> SPLQAKKVR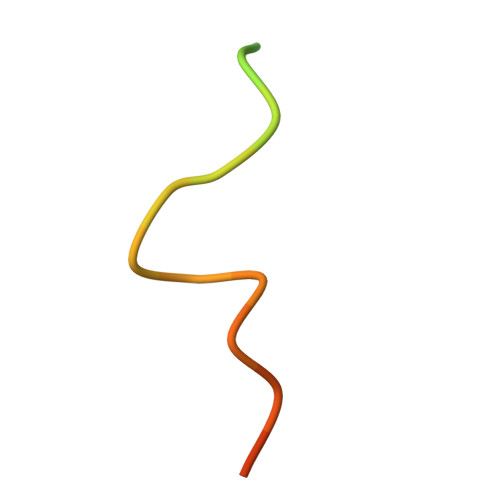KVPPGLPSSVYAPSPN>HMPALLKRLLFQVGPHPNERTFTLSSVSTDGHYISLRPFVKPSGDELSFPFEWAFAGTNETVKANDQGNGVVTQDFNFWLDTNVYLNVPNTHRGEVNTTWKNWDSGCVEETGAVYPFGADKESVSFREMWQPVDPSREDLVIVSPNNEKFSSNARSIVLKVTDEAYDGLVIVIGRWI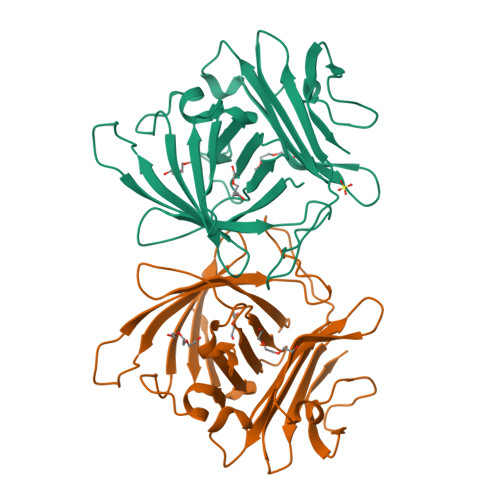QGFLSQKNNNTIEGLNFIRLLEKDSGKSEFLLSYGKEVNKIPQSYENLKKGSTVTSNGLNWEVIEYHA[2x]>[4x]KMERKNVWHHRKKEEIEAFSKEYMEF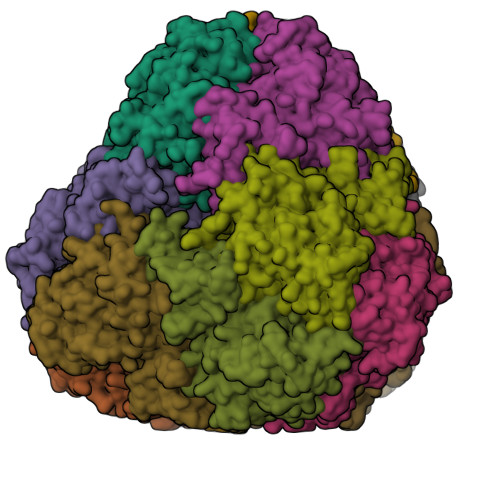MSKAKTERMTVKEIKRILDESGFVPLEDFAGDPMNMTVYAVNRGKAIAAFRVVDDLKRGLNLVVAHIDSPRLDFKPNPLIEDEQIALFKTHYYGGIKKYHWLSIPLEIHGVLFKNDGTEIEIHIGDKPEDPVFTIPDLLPHLDKEDAKISEKFKGENLMLIAGTIPLSGEEKEAVKTNVLKILNEMYGITEEDFVSGEIEVVPAFSPREVGMDRSLIGAYGQDDRICAYTALRALLSANPEKSIGVIFFDKEEIGSDGNTGAKARFYLKALRQILKMQGAKDSEFVLDEVLENTSVISGDVCAAVNPPYKDVHDLHNAPKLGYGVALVKYTGARGKYSTNDAHAEFVARVRKVLNEQGVIWQVATLGKVDQGGGGTIAKFFAERGSDVIDMGPALLGMHSPFEISSKADLFETYVAYRSLMEKL Potassium‐coupled chloride transporters (KCCs) play crucial roles in regulating cell volume and intracellular chloride concentration. They are characteristically inhibited under isotonic conditions via phospho‐regulatory sites located within the cytoplasmic termini. Decreased inhibitory phosphorylation in response to hypotonic cell swelling stimulates transport activity, and dysfunction of this regulatory process has been associated with various human diseases. Here, we present cryo‐EM structures of human KCC3b and KCC1, revealing structural determinants for phospho‐regulation in both N‐ and C‐termini.

To gain further insights into the structure KCCs in an activated, non‐phosphorylated state, we took advantage of an N‐terminally deleted variant of the closely related KCC1 transporter (KCC1Δ19) with deleted N‐terminal OSR‐1‐binding motif H/RFXV (residues 3‐6 in full‐length KCC1 (Austin et␣al, 2014)). Interestingly, 3D classification of the KCC1Δ19 dataset yielded two conformations that differ mainly in the degree of the counter‐clockwise CTD twist and the inter‐subunit distances between the central TM11/12 helices. The coexistence of two alternating CTD conformations in KCC1Δ19 is indicative of an increased flexibility around the TM‐CTD‐connecting scissor helices compared to KCC3b‐PM. Helix α8 moves from a position close to the central β‐sheet to a position further away from the TM region, over a distance of 30.6 Å (Cα–Cα distance of T926 in state 1 and state 2), by undergoing a 47° rotation around the β7 strand. In these two alternative conformations, α8 is either located above or below the α10 helix. The first state of the α8 helix close to the centre of CTD resembles our KCC3b‐PM structure and the structure of wild‐type KCC3b published by another group while this work was under review (Chi et␣al, 2020). Inspection of the electron density in this region of the KCC1 map suggests that either ADP or ATP are bound to the Rossmann‐like fold formed by β‐strands β1, β2 and β4 and helices α1, α3, α4 of the KCC1 inner lobe. Weaker density for the γ‐phosphate indicates that a mixture of ADP‐ and ATP‐bound particles may contribute the observed densities (Fig EV4A).

>MLEGLSWVDYGERAELDDSDGHGNHRESSPFLSPLEASRGIDYYDRNLALFEEELDIRPKVSSLLGKLVSYTNLTQGAKEHEEAESGEGTRRRAAEAPSMGTLMGVYLPCLQNIFGVILFLRLTWMVGTAGVLQALLIVLICCCCTLLTAISMSAIATNGVVPAGGSYFMISRSLGPEFGGAVGLCFYLGTTFAAAMYILGAIEILLTYIAPPAAIFYPSGAHDTSNATLNNMRVYGTIFLTFMTLVVFVGVKYVNKFASLFLACVIISILSIYAGGIKSIFDPPVFPVCMLGNRTLSRDQFDICAKTAVVDNETVATQLWSFFCHSPNLTTDSCDPYFMLNNVTEIPGIPGAAAGVLQENLWSAYLEKGDIVEKHGLPSADAPSLKESLPLYVVADIATSFTVLVGIFFPSVTGIMAGSNRSGDLRDAQKSIPVGTILAIITTSLVYFSSVVLFGACIEGVVLRDKYGDGVSRNLVVGTLAWPSPWVIVIGSFFSTCGAGLQSLTGAPRLLQAIAKDNIIPFLRVFGHGKVNGEPTWALLLTALIAELGILIASLDMVAPILSMFFLMCYLFVNLACAVQTLLRTPNWRPRFKYYHWALSFLGMSLCLALMFVSSWYYALVAMLIAGMIYKYIEYQGAEKEWGDGIRGLSLSAARYALLRLEEGPPHTKNWRPQLLVLLKLDEDLHVKYPRLLTFASQLKAGKGLTIVGSVIQGSFLESYGEAQAAEQTIKNMMEIEKVKGFCQVVVASKVREGLAHLIQSCGLGGMRHNSVVLGWPYGWRQSEDPRAWKTFIDTVRCTTAAHLALLVPKNIAFYPSNHERYLEGHIDVWWIVHDGGMLMLLPFLLRQHKVWRKCRMRIFTVAQMDDNSIQMKKDLAVFLYHLRLEAEVEVVEMHNSDISAYTYERTLMMEQRSQMLRQMRLTKTEREREAQLVKDRHSALRLESLYSDEEDESAVGADKIQMTWTRDKYMTETWDPSHAPDNFRELVHIKPDQSNVRRMHTAVKLNEVIVTRSHDARLVLLNMPGPPRNSEGDENYMEFLEVLTEGLERVLLVRGGGREVITIYSAENLYFQ[2x]~{N}-(4-chlorophenyl)-2-cyano-ethanamide | C9 H7 Cl N2 O | 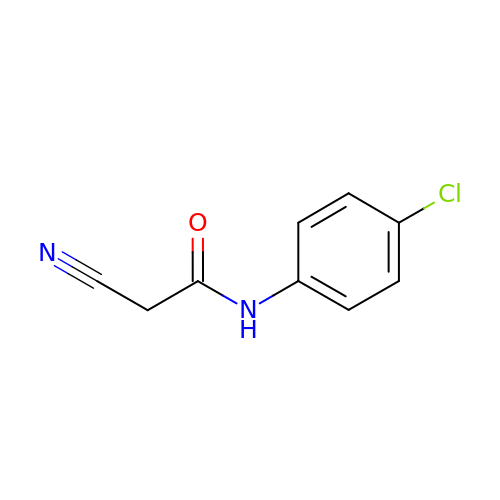FLLVVAHFEBGZKD-UHFFFAOYSA-N>[2x]MHHHHHHSSGRENLYFQGMPKEYGADSITILEGLEAVRKRPGMYIGSTGERGLHHLIWEVVDNAVDEAMAGFATRVDVKIHADGSVEVRD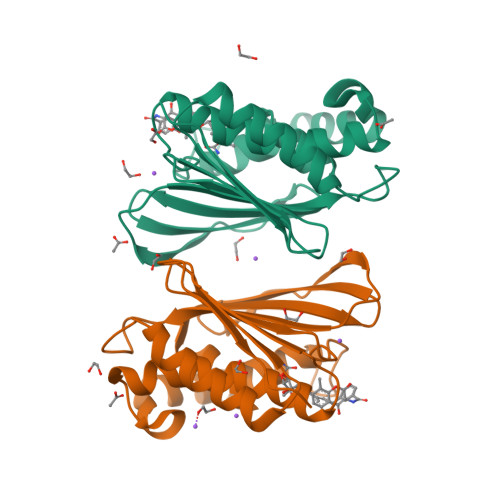DGRGIPVEMHATGMPTIDVVMTQLHAGGKFDGETYAVSGGLHGVGVSVVNALSTRLEATVLRDGYEWFQYYDRSVPGKLKQGGETKETGTTIRFWADPEIFETTDYNFETVARRLQEMAFLNKGLTIELTDERDGKHRVFHYPG>MSNSAIPLNVVAVQEPRLELNNERTWVVVKGGQQVTYYPFPSTSFSSNQFNFICNPPSAQTVLDRLVFIQVPYDITFTANPSHAGITENLLQP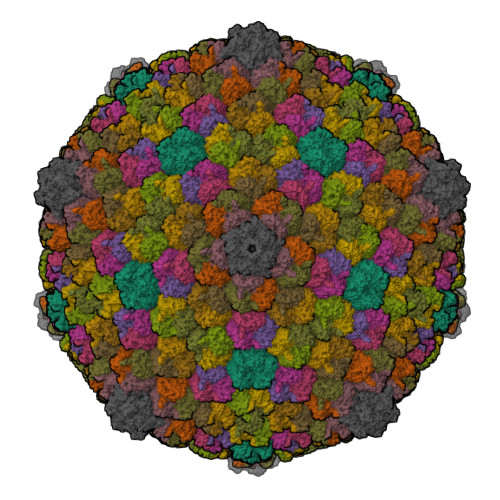GRDAFRAFPISSITNTLNATINGFPVNIELAQIIHALSRYHTPLKVKNGWMSMQPSFEDNYQSYRDADGANNNPLGVFTSAAGLSELPRGSYTMNVVTNTTTTARITGVLYEQVFLPPFLWDGEQAGGLANLTSLTFNWVLNNNLARIWSHSDITNDVSGNSTIGSMNISFQQPSMYLGFVTPRLNIPIPPRITYPYFKLSRYTTQFQNTLAPNASSTFKSNVVQLDSIPRKLYLFVKQSDNVIYQNLNNQITTPDVFLQINNLNLTWNNQQGILSGASSQNLYDFSVQNGYNKTWSEFNGVTQQFNGVSGQPTKVIGLEGGIVCLELGKDVGLRDDEAEGVIGNFNLQVQMTVTNTNQYVTVTPDMYIVAVYDGTLVISNTSAMASIGVASKEEVLNARITHGVSYNELQRIYG[13x];> MSYSHSIKDCQEPDTVYYDILIPFKPNDQGFSPAIFQAQLTQPIVHNPSEYFLSVVRFSIPTQNIPLTIPQIQPYPNTNVNNTIYSVSIGYNGTYSSQNFVQFDPSLTSPNIPAPNAPTVTSPNVEVTPYYYIYDYSTFLQMINTALENAFNEISAPVGADAPFFFYDSNTEKISLIAQAAYYDRTLTTPIEIYCNVNLFTFFDSIKHIGLGYNTPTGRDILFDVRFLGNNYYQDPETAPSYPPEFIQMQQEYPTLSNWNAVKTIQLVSNLLPINKESIPSFRNSNVGIINAQGILADFVPLVTNGPEARISIDFVATGPWRLIDMFGSVPIYMVDLYVYWTDQTGGQYLINIPPGRILTCKLVFIKKSLSKYLVSEK> MSALPPVYSFPPLYTRQPNSLTRRQQISTWIDIISQYCKTKKIWYMSVDGTVINDNELDSGSTDNDDSKKISKNLFNNEDIQRSVSQVFIDEIWSQMTKEGKCLPIDQSGRRSSNTTTTRYFILWKSLDSWASLILQWFEDSGKLNQV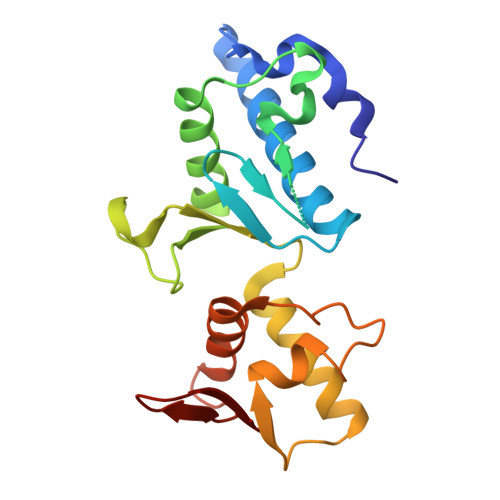ITLYELSEGDETVNWEFHRMPESLLYYCLKPLCDRNRATMLKDENDKVIAIKVV> SNNVLPTWSLDSNGEMRSRLSLSEVLDSGDLMKFAVDKTGCQFLEKAVKGSLTSYQKFQLFEQVIGRKDDFLKLSTNIFGNYLVQSVIGISLATNDDGYTKRQEKLKNFISSQMTDMCLDKFACRVIQSSLQNMDLSLACKLVQALPRDARLIAICVDQNANHVIQKVVAVIPLKNWEFIVDFVATPEHLRQICSDKYGCRVVQTIIEKLTADSMNVDLTSAAQNLRERALQRLMTSVTNRCQELATNEYANYIIQHIVSNDDLAVYRECIIEKCLMRNLLSLSQEKFASHVVEKAFLHAPLELLAEMMDEIFDGYIPHPDTGKDALDIMMFHQFGNYVVQCMLTICCDAVSGRRQTKEGGYDHAISFQDWLKKLHSRVTKERHRLSRFSSGKKMIETLANLRSTH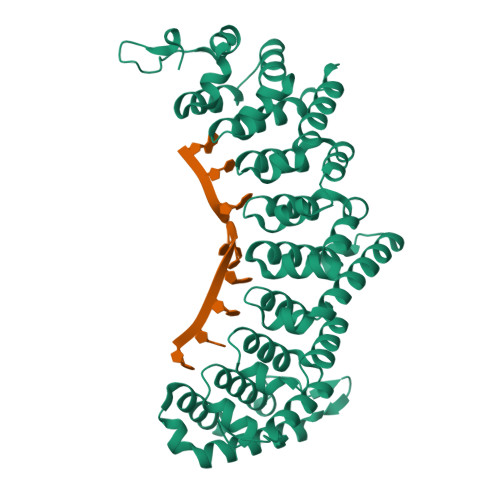PIYELQ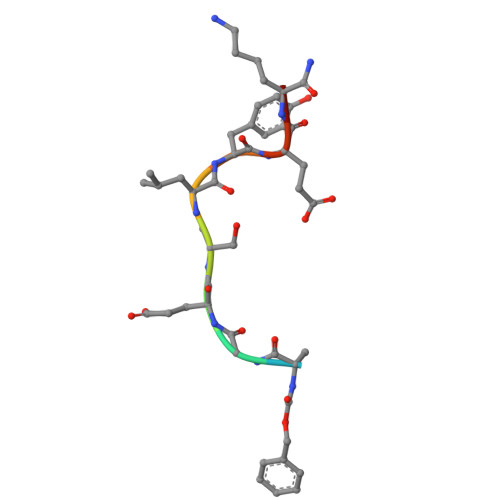> XAGESLYEKX>[2x]GSHMLDGCTPWPAEFAVRYREAGYWTGETFSDFVTDRTRRFADRLAVVGAGQRWTYAELGERSAVLATGLARLGIAAGDRVVVQLPNIPELFEVVFALFRLGALPVYALPAHRAHEITHLCTTAQAKALIIPDRHAGFDYRTMAAQLRHAGTAPEHVVVVGEPGGFTPLAELRADRPDPGVFTRPEASDAAFLQLSGGTTGLPKLIPRTHDDYLYSVRASAEICALGTDTVYLAALPAVHNFPMSSPGFLGTFHAGGTVVLAPNPSPDTAFSLIETERVTITAVVPPIALQWLDAVEHGSQSHRDLSSLRVLQ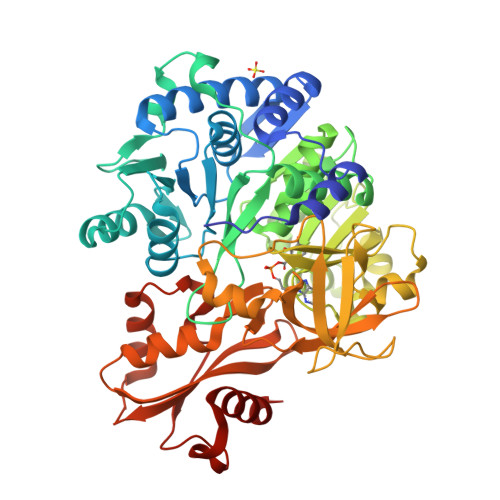VGGAKFAPEAARRVRPVLGCTLQQVFGMAEGLVNYTRLDDPDDIITTTQGRPISPDDEIRIVDEADRPVPDGEVGHLLTRGPYTIRGYYRAEEHNATAFTPDGFYRTGDLVRRTPTGHLVVEGRAKDQINRGGEKVSAEEVENHILAHPAVHDAAVVGMSDPYLGERVCAYVIARTEPPSRSELLRFLRERGLASYKIPDRVEFVDRFPVTGVGKISRSELRRELARRLDTTR>GSHMMIYPDEAMLYAPVEWHDCSEGFEDIRYEKSTDGIAKITINRPQVRNAFRPLTVKEMIQALADARYDDNIGVIILTGAGDKAFCSGGDQKVRGDYGGYKDDSGVHHLNVLDFQRQIRTCPKPVVAMVAGYSIGGGHVLHMMCDLTIAADNAIFGQTGPKVGSFDGGWGASYMARIVGQKKAREIWFLCRQYDAKQALDMGLVNTVVPLADLEKETVRWCREMLQNSPMALRCLKAALNADCDGQAGLQELAGNAT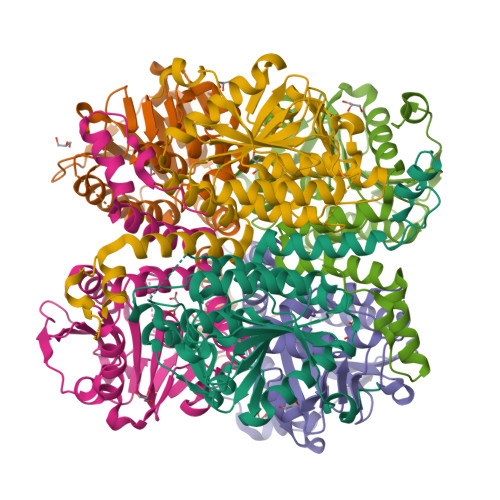MLFYMTEEGQEGRNAFNQKRQPDFSKFKRNP[6x]> MHHHHHHHHHHGENLYFQGSDNIISFDHVTFTYPDSPRPALSDLSFAIERGSWTALIGHNGSGKSTVSKLINGLLAPDDLDKSSITVDGVKLGADTVWEVREKVGIVFQNPDNQFVGATVSDDVAFGLENRAVPRPEMLKIVAQAVADVGMADYADSEPSNLSGGQKQRVAIAGILAVKPQVIILDESTSMLDPEGKEQILDLVRKIKEDNNLTVISITHDLEEAAGADQVLVLDDGQLLDQGKPEEIFPKVEMLKRIGLDIPFVYRLKQLLKERGIVLPDEIDDDEKLVQSLWQLNSKM;> MAIKFENVSYVYSPGSPLEAIGLDQLNFSLEEGKFIALVGHTGSGKSTLMQHFNALLKPTSGKIEIAGYTITPETGNKGLKDLRRKVSLAFQFSEAQLFENTVLKDVEYGPRNFGFSEDEAREAALKWLKKVGLKDDLIEHSPFDLSGGQMRRVALAGVLAYEPEIICLDEPAAGLDPMGRLEMMQLFKDYQAAGHTVILVTHNMDDVADYADDVLALEHGRLIKHASPKEVFKDSEWLQKHHLAEPRSARFAAKLEAAGLKLPGQPLTMPELADAIKQSLKGGEHE;> MKSESKVSSKLELRELVLLAMVIAIKVILGQFKVGNATLQVGLGFIGSVMLGYLFGPWWGFAGGALSDLVSSVIFGNLGGFFIGFTLTAALGPMIYGFFLYKQPIQIWRVIASVICVTVICNIGLNTLWVSMMYGINFMVALSSRILKEMITPWIQMVAVWFILEGLSRVKLSRKFWSHPQFEK;> MSKIIIGRYLPGTTFVYRVDPRAKLLTTFYFIIMIFLANNWVSYLVISIFGLAYVFATGLKARVFWDGVKPMIWMIVFTSLLQTFFMAGGKVYWHWWIFTLSSEGLINGLYVFIRFAMIILVSTVMTVTTKPLEIADAMEWMLTPLKLFKVNVGMISLVISIALRFVPTLFDQTVKIMNAQRSRGADFNDGGLVKRAKSVVPMLVPLFIDSLEVALDLSTAMESRGYKGSEGRTRYRILEWSKVDLIPVAYCLLLTILMITTRKH

Energy-coupling factor (ECF)-type transporters mediate the import of micronutrients, such as folate, cobalamin and pantothenate, in the majority of prokaryotes. A tripartite ATP-hydrolysing motor (ECF module), composed of a membrane-embedded scaffold protein (EcfT) and two cytosolic nucleotide-binding proteins or ATPase subunits (often hetero-dimeric - EcfA and EcfA’), forms a functional core complex with a membrane-embedded substrate-translocating protein (S-component). Structural and biophysical analyses of ECF transporter complexes from three different organisms, with different substrate specificities, and from different laboratories revealed that the core complex and minimal functional unit exists in a 1:1:1:1 subunit stoichiometry. Based on these fragmented structural insights, a model for the transport mechanism has been proposed in which a substrate-free solitary S-component with an outward-facing binding site topples within the membrane upon substrate acquisition, associates with the ECF module, and exposes the binding site to the cytosol, thereby moving the substrate across the membrane.

Accordingly, we incubated ECF-FolT2 with Mg-ATP and folate prior to sample vitrification. The S-component for folate (FolT2) remains docked to the EcfT subunit in the substrate-free inward-facing toppled state. The ATPase dimer adopts the open conformation, albeit with bound nucleotides. The nucleotides interact only with motifs from a single ATPase subunit and are separated from the signature motif (LSGGQ) located in the other ATPase. Notably, the nucleotide occupancy in the nucleotide-binding sites of ECF-FolT2ATP is asymmetric with ATP and ADP bound to the EcfA and EcfA’ subunits, respectively, which has been also observed in other ABC transporters. ADP is bound exclusively by residues from the EcfA’ subunit, and its presence suggests that ATP hydrolysis had occurred. In contrast, ATP remained present in the EcfA subunit, where the adenine moiety of ATP is sandwiched through π-interactions between Phe13 in the EcfA subunit and Arg174 in the carboxy-terminal end of the S-component FolT2. An indication from such asymmetry comes from the structure of the nanodisc-reconstituted full complex ECF-FolT2ATP determined here in the presence of ATP, resembling turnover conditions. Intriguingly, this structure adopts an open conformation, but where ATP hydrolysis has occurred only in one of the sites, while ATP remained associated with the second site, and was apparently protected from hydrolysis. We speculate that the S-component, which remains associated with the ECF module in the nanodisc environment, hinders the conformational transition needed for hydrolysis of the second ATP molecule.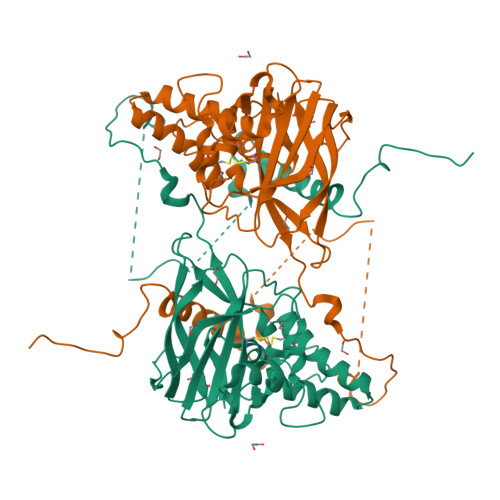> HGYITFPIARQRRCNVQGGFWWPPDGSGIPDPMCRAAYQNVYNKVLQQGGTIDQAASAAQYMFQQDNEYAALAGPNYLDQNHIRNNVVPNYLCAAHATTWRIRPFGDKTGMDVSGSWTPTVIPLQDNTVSTVPIEFEFCPTAIHEPSFFEIYITVPSFNVYTDQVTWQQLINIFTGPIPLVQRRPDSQCNANNLVYRTTVGIPVRQTQFVLYVRWQRNDPVGEGFYNCADVIFAHRLGINEEDKIRPPKMKCKGNDKDCYKHHHRHNRYENDYENNYENYENYENNYENNYENNYENNYEYEYEYDRNNREHYHKCKHHSCMQHNYYERQYNTKDFNYVEWNDDYSDYIENHTGINRDMCDSTTKCCYKK> MKIYQKRLEYYTDSRDYDNLRSLSPLSDSSVNKSPEEHKQDAESEKNLKNINPDYRFWIKVEGTNIDFPVVQGKDNDFYLHHNFNKEKSFSGSIFVDSENNLNDDSNIVVYGHNMRNDTMFAQIKHFKNENFFNANKYVTLYREGKKSTFEIFSVYQENAKDLESEIKT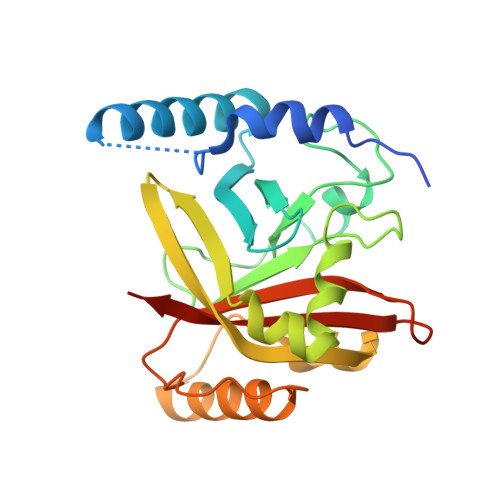KFSNKEDYEKYLKEQESKSLFKRDGIDLNSNDRILTLITSGYDFVNARIVVVAKEIDLEHHHHHH>MLVSVYLALLVACVGQAHSQANLMRLKSDLFNRSPMYPGPTKDDPLTVTLGFFLQDIVKVDSSTNEVDLVYYERQRWKLNSLMWDPNEYGNITDFRTSAADIWTPDITAASSTRPVQVLSPQIAVVTHDGSVMFSPAQRLSFMCDPTGVDSEEGVTCAVKFESWVYSGFEIDLKTDTDQV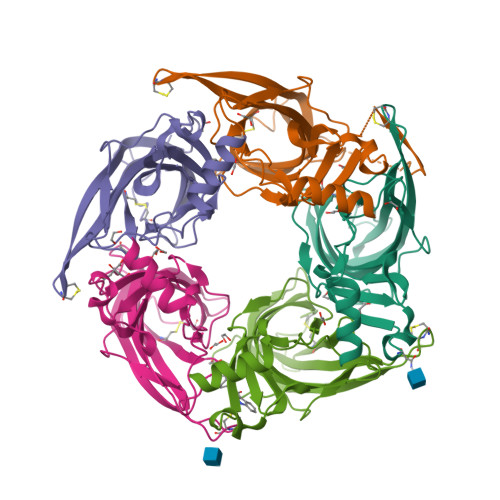DLSSYYASSKYEILSATQTRQVQHYSCCPEPYIDVNLVVKFRERRAGNGFFRNLFDENLYFQGHHHHHH[10x]>[6x]MKIINARLRRQEALFTLDLQDGIIHRITAQAAMQTADAGAIDAQGRLAIPPFVEPHIHLDATLTAGEPEWNRSGTLF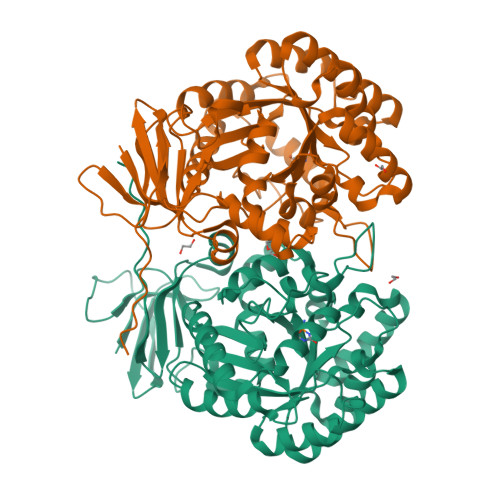EGITRWSQRKASITPEDTRQRALKTIGMLRDFGVQHVRTHVDVTDPSLAALQALLAVKQEAADLIDLQIVAFPQEGIESYPNGRELMTRAIEMGADVVGGIPHYENTRDKGVSSVMFLMDLAQRYGRLVDVHCDEIDDPQSRFLEVLAEEARVRGMGAQVTASHTCAMGSYDNAYCSKLFRLLKASGINFISCPTESIHLQGRFDSWPKRRGVTRVAELDRAGINVCFAQDSIQDPWYPLGNGNILRILDAGLHICHMLGYDDLQRCLDFVTDNSARALCLGDNYGLAEGRPANLLILDAENDYEAVRRQARVLTSIRHGKVILQREVEHIRYPANSSSVDKLAAALEHHHHHH> SNSLNILDDDYNGQAKCMLEKVGNWNFDIFLFDRLTNGNSLVSLTFHLFSLHGLIEYFHLDMMKLRRFLVMIQEDYHSQNPYHNAVHAADVTQAMHCYLKEPKLANSVTPWDILLSLIAAATHDLDHPGVNQPFLIKTNHYLATLYKNTSVLENHHWRSAVGLLRESGLFSHLPLESRQQMETQIGALILATDISRQNEYLSLFRSHLDRGDLCLEDTRHRHLVLQMALKCADICNPCRTWELSKQWSEKVTEEFFHQGDIEKKYHLGVSP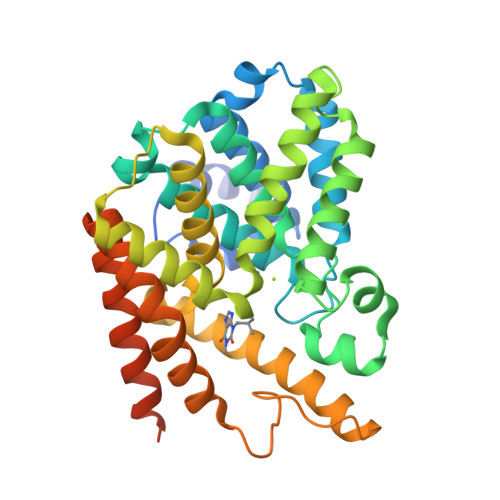LCDRHTESIANIQIGFMTYLVEPLFTEWARFSNTRLSQTMLGHVGLNKASWKGLQREQSSSEDTDAAFELNSQLLPQENRLS>[2x]GPHMGEEAPPGVRSVKVVLVGDGGCGKTSLLMVFADGAFPESYTPTVFERYMVNLQVKGKPVHLHIWDTAGLDDYDRLRPLFYPDASVLLLCFDVTSPNSFDNIFNRWYPEVNHFCKKVPIIVVGCKTDLRKDKSLVNKLRRNGLEPVTYHRGQEMARSVGAVAYLECSARLHDNVHAVFQEAAEVALSSR;>[2x]EYAPLTVSVIVQDEGIDAIPVKVLNCDTISQVKEKIIDQVYRTQP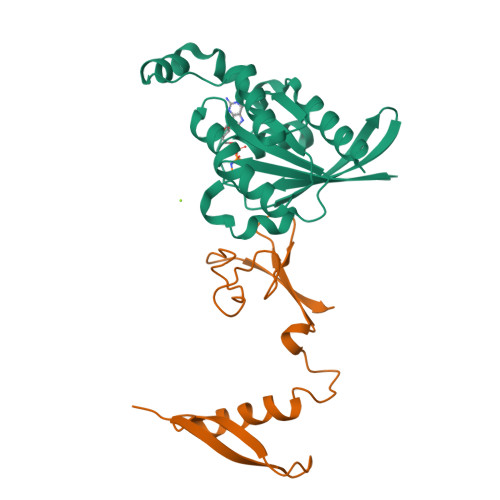CSCWPKPDSVVLEWRPGSTAQILSDLDLTSQREGRWKRINTLMHYNVRDGATLILSKV>MPPETATNPKDARHDGWQTLKRFLPYLWPADNAVLRRRVVGAILMVLLGKATTLALPFAYKKAVDAMTLGGGAQPALTVALAFVLAYALGRFSGVLFDNLRNIVFERVGQDATRHLAENVFARLHKLSLRFHLARRTGEVTKVIERGTKSIDTMLYFLLFNIAPTVIELTAVIVIFWLNFGLGLVTATILAVIAYVWTTRTITEWRTHLREKMNRLDGQALARAVDSLLNYETVKYFGAESREEARYASAARAYADAAVKSENSLGLLNIAQALIVNLLMAGAMAWTVYGWSQGKLTVGDLVFVNTYLTQLFRPLDMLGMVYRTIRQGLIDMAEMFRLIDTHIEVADVPNAPALVVNRPSVTFDNVVFGYDRDREILHGLSFEVAAGSRVAIVGPSGAGKSTIARLLFRFYDPWEGRILIDGQDIAHVTQTSLRAALGIVPQDSVLFNDTIGYNIAYGRDGASRAEVDAAAKGAAIADFIARLPQGYDTEVGERGLKLSGGEKQRVAIARTLVKNPPI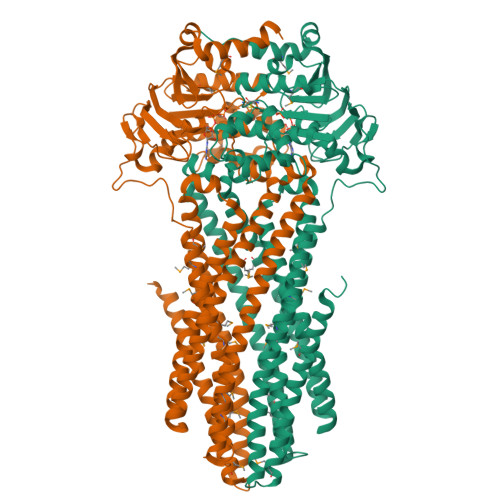LLFDEATCALDTRTEQDILSTMRAVASHRTTISIAHRLSTIADSDTILVLDQGRLAEQGSHLDLLRRDGLYAEMWARQAAESAEVSEAAEHHHHHH[2x]2-(DIMETHYLAMINO)ETHYL (1Z)-2-PHENYL-N-(SULFOOXY)ETHANIMIDOTHIOATE 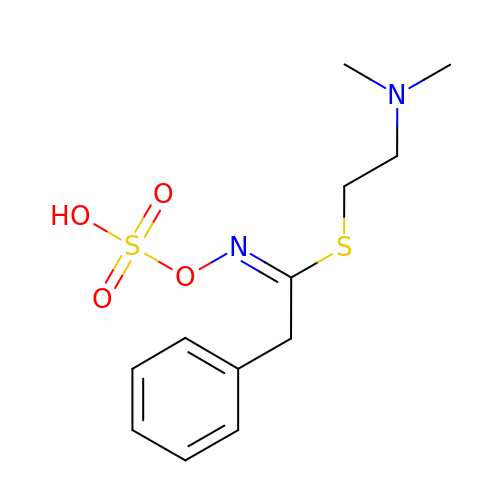| C12 H18 N2 O4 S2 | AJWBDCAFLSUABV-SEYXRHQNSA-N> PLPWCPHLVAVCPIPAAGLDVTQPCGDCGTIQENWVCLSCYQVYCGRYINGHMLQHHGNSGHPLVLSYIDLSAWCYYCQAYVHHQALLDVKN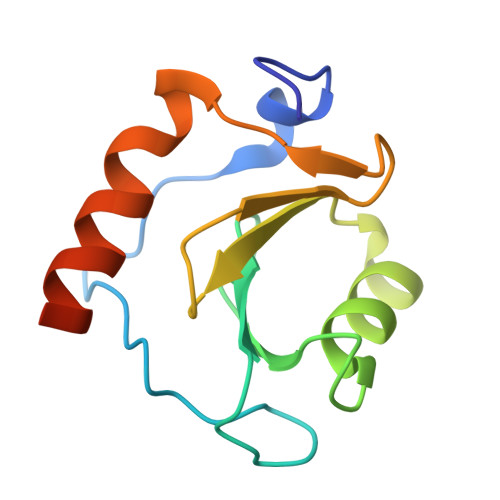IAHQNKFGEDMPHPH>[2x]MFKYVIPLCALTLAAPSFAAQTTLMLSQKSDVNYLGWSTDESKVARQEVYRGTTSNPDLRERIAVLDAETRTFKDADTNSGLNYWYWVDVVSENQAQVVSNAVTTAPNAGPLRAAKASSECKPGATFENRTVDCGGVTIGTSCPNDSDKQKPLIILKNATVKNLRISASGGADGIHCDSGNCTIE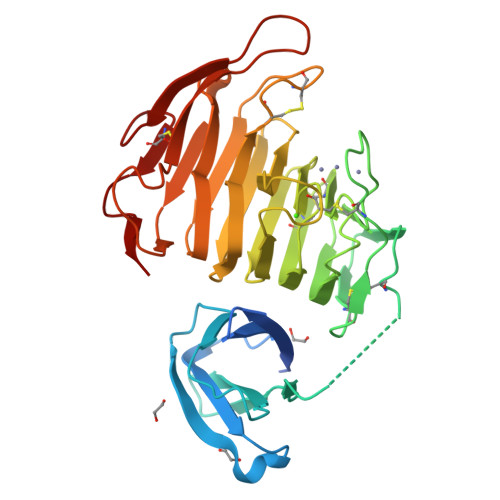NVIWEDICEDAATNNGKTMTIVGGIAHNAKDGYGGKPDKVLQHNSKNSTTVVKGNFTLTGEHGKLWRSCGDCSNNGGPRFLTVTSATVNGTIDSIAGVNRNYGDVATISGLKIKNYKEGKPPVCEEFKGVVKGQGSTEKYGEKWDTTNCKVSRSGVSKL>AAVLQQVLERTELNKLPKSVQNKLEKFLADQQSEIDGLKGRHEKFKVESEQQYFEIEKRLSHSQERLVNETRECQSLRLELEKLNNQLKALTEKNKELEIAQDRNIAIQSQFTRTKEELEAEKRDLIRTNERLSQEL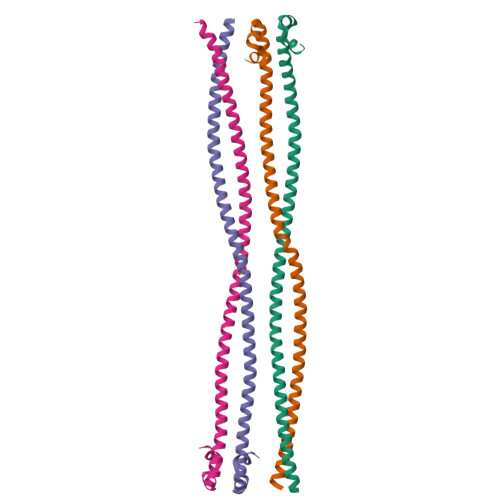EYLT[4x]We report structures of the Mycobacterium tuberculosis isoprenyl diphosphate synthase Rv2173 in three forms: apo and two substrate-bound forms [isoprenyl diphosphate (IPP) and dimethylallyl diphosphate (DMAPP)]. The protein possesses a canonical all-α-helical trans-isoprenyl diphosphate synthase fold that is dimeric in each form. Two divalent-metal-binding aspartic acid-rich DDxxD motifs termed the FARM and SARM (first and second aspartic acid-rich DDxxD motifs) are important in all-E-prenyltransferase mechanisms. Rv2173 is a homodimer with a canonical class I diterpene synthase fold, with structural analysis identifying some conserved mechanistic features in C-terminal closure and supporting its annotation as a short-chain (C10–C15) product-length synthase.

The apo structure was solved with a dimer in the asymmetric unit in space group P21212, while both substrate-bound structures were solved in space group I222 with monomers in the asymmetric unit, generating dimers on the application of crystallographic symmetry. Consistent with most E-prenyltransferases, which exist as homodimers or heterodimers, Rv2173 is a dimer in the crystal structure, with this biological assembly supported by native mass spectrometry. All three structures are very similar (0.36–0.65 Å r.m.s.d. across all Cα atoms as calculated by SSM; Krissinel & Henrick, 2004), with the main variation being in the completeness of the C-terminus; the apo structure is missing the last four residues and the DMAPP-bound structure the last eight residues, while the IPP-bound structure has a complete C-terminus. It is these C-terminal residues in conjunction with the aforementioned lid helices that are likely to close the active site fully during the reaction cycle. There are some differences between the structures: the IPP-bound form shows IPP bound in the DMAPP/allylic substrate-binding site with three divalent metal ions bound around the IPP and the complete C-terminus closing around the active site, while the apo and DMAPP-bound forms are more open, with some of the C-terminal region disordered, supporting suggestions that the C-terminus is important in substrate entry/product exit. In no case is the IPP binding site occupied by IPP. Additionally, in all structures, and even in this most closed form, the basic residue Lys43, which is likely to be important for the binding of the PP group in the IPP site, is poorly ordered and this disorder may also influence variability in positioning of the metal ions.

>[2x]MSYYHHHHHHLESTSLYKKAGSAAALFRFKKEPFTMAGAITDQLRRYLHGRRRAAAHMGSDYDGLIADLEDFVLGGGKRLRPLFAYWGWHAVASREPDPDVLLLFSALELLHAWALVHDDLIDRSATRRGRPTAQLRYAALHRDRDWRGSPDQFGMSAAILLGDLAQVWADDIVSKVCQSALAPDAQRRVHRVWADIRNEVLGGQYLDIVAEASAAESIESAMNVATLKTACYTVSRPLQLGTAAAADRSDVAAIFEHFGADLGVAFQLRDDVLGVFGDPAVTGKPSGDDLKSGKRTVLVAEAVELADRSDPLAAKLLRTSIGTRLTDAQVRELRTVIEAVGARAAAESRIAALTQRALATLASAPINATAKAGLSELAMMAANRSA> GSQFTDVKCTGSKQCWPVCKQMFGKPNGKCM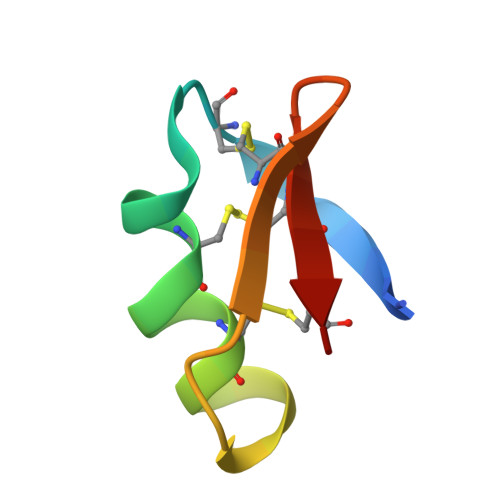NGKCRCYS>[2x]AMNTVLELQKLAHD;>NMLYHRYLKPNSEYYKKIEVRGKDNIYELNDIPDTYAVFLDNESVWKHYHVKGSTLPEQGWKIHVTSSLEDSKDVLDKVARLCIDKKIEFKHLKDKDSFMKMNSKNANRASSGKFITIYPTNNEVFVELLEMISLAIQDFKKGPYILNDKRWKNSNVFYRYGGFKGIFNEHGEHCIRDKEGNLIKDQRNPFYQVPDFVKDFDDYLNTINNSGELENKGESRLGKYKIETALSFSNAGGVYLATRKKDNLKVIIKEARPSAGLDGAAQDALARQKIEYDALKKLKDVSGVVNLIEYFQEWEHYFLVEEFIEGRDLRQWIAQEFPFFEDNNGMSNHIKDVKMILLQLLDLIDSMHNQGVAMGDLQPANIMVTEDLTVRIIDFETAMPVNSDDRPAMLTTGFVSHEMKVSGARDWFGFKRLVRYLALPVLTSEDLEGYLQYNHLNWIKENYGYEFYSFIVDLQEKCDKRIKDYQTFIPKEINLNDQTSDFNLTSIINKLIIGVESSLTNDERFINGDIRQFEMNGGKFNFLTGGSGAAFTLTKNKSSIAEVDKWIQSVLLDNLPLIEEDGLFTGKTGILALLYDKGYKEVVLNELKILKDNINQTDISIRSGLSGIGLFVISLYLETENKEYLKLAKDLERMIKLNRAKDKQLKVKDWMAVDIGVIDGLSGVSLFYSALYSVTQNQKYLEEAEVLIKEDLESTKKDDVTGVLQTVDNKNRLLPYLSGGSIGVAISIWFLNHVSGQDLYREEMNSILKLSKTRCTISGGLFDGAGSFLLIPSMVKNDKNREVILNEVLNLLNIFLIEKNSYYVYPGQFSYRLADDVYTGSSGIILALMGVIKGNPLYWLPLVNSDEFLARTKV[2x]

In bacteria, Ser/Thr protein kinase-like sequences are found as part of large multidomain polypeptides that biosynthesize lanthipeptides, a class of natural products distinguished by the presence of thioether cross-links. The kinase domain phosphorylates Ser or Thr residues in the peptide substrates. Subsequent β-elimination by a lyase domain yields electrophilic dehydroamino acids, which can undergo cyclase domain-catalyzed cyclization to yield conformationally restricted, bioactive compounds. We also describe the first crystal structures of a class III lanthipeptide synthetase, consisting of the lyase, kinase, and cyclase domains, in various states including complexes with its leader peptide and nucleotide.

Leader peptide residues Asp(−10) to Met(−22) are bound perpendicular to the antiparallel β-strands that form the N-lobe of the kinase domain. A comparison with the structure of wild-type ThurKC bound to the leader peptide in trans (2.45 Å resolution) confirms the binding mode and rules out artifactual binding due to the single-chain fusion. The leader region binds as a three turn α-helix, encompassing residues Lys(−14) through Met(−22), and the helical configuration is consistent with prior multidimensional NMR studies of the synthetic leader peptides of class III lipolanthine from M. arborescens (MicA from the microvionin pathway). The remainder of the leader sequence (Leu(−13) through Asp(−10)) exists in an extended form and is directed toward the kinase and lyase active sites. The leader helix is amphipathic in nature with the hydrophobic residues directed toward contacts with the ThurKC and most of the polar residues facing toward the solvent. The leader binding groove in ThurKC is formed by several aromatic or aliphatic residues from both the kinase and the lyase domains that provide van der Waals contact with the peptide. The last of the helical residues from the leader that contacts the protein is Gln(−15), and this residue is engaged in hydrogen bonding interactions with Tyr243 and Glu258 from the kinase domain and Arg112 from the lyase domain. Notably, an aromatic residue located at the very start of the kinase domain (Phe236) disrupts the helical configuration, resulting in the remainder of the leader being extended as a coil that may enable shuttling between the different actives sites of ThurKC. The structures of ThurKC bound to the leader peptide, either as a single-chain fusion or in trans, identify the correct binding site for the leader in a class III system, which is distinct from previously predicted models. Comparison of the ThurKC structure in the absence and presence of the leader peptide demonstrates that leader binding orients interactions between all three domains.> EKEKKNVFMRTFEAISRNFSEIFAKLSPGGSARLILENPEDPFSGGLEIEAKPAGKDVKRIEAMSGGEKALTALAFVFAIQ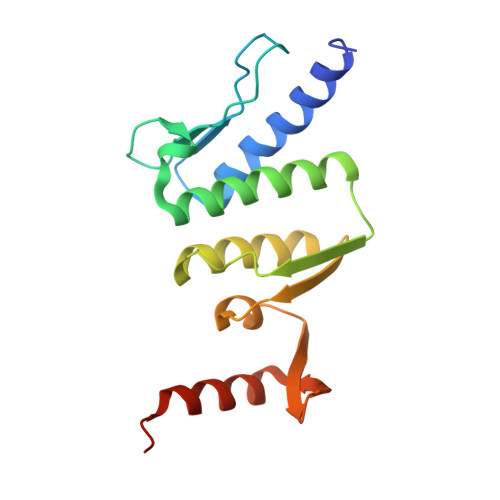KFKPAPFYLFDQIDAHLDDANVKRVADLIKESSKESQFIVITLRDVMMANADKIIGVSMRDGVSKVVSLSLEKAMKILEEIRKKQGWEHGN>MIFRQLFDSESSTYTYLIGDEATRQAVLIDPVLEQVDRDLQMVAELDLTLTHVFDTHVHADHITASGALRER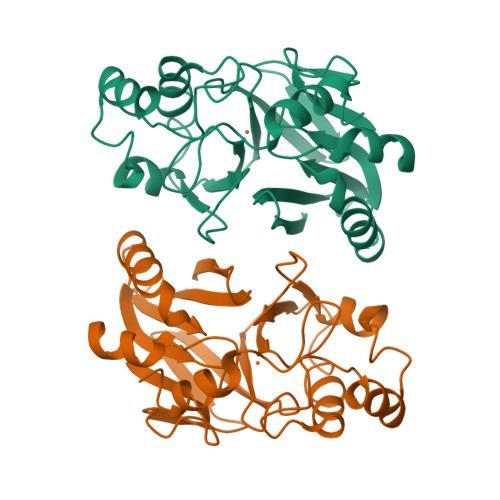TQATVVGSVNGASCANVQVRHGDEVRVGQLVFQVLATPGHTDDSISYLLGDRVFTGDALLVRGNGRTDFQNGNASQLYDSLTRVLFTLPDETLVYPGHDYKGRTVTSIAEEKRHNPRVAGKSREEFIHIMENLNLPRPKLIDAAVPANRACGHTAPSPQGA[2x]>[2x]MKLALNTEFKKAIDLATNSSKNLFITGKAGTGKSTFLKYLINELLFDAVVLAPTGVAAINIGGETIHSFFNFPINITPDKIPDLFIYDYEIYKYVNTIIIDEISMVRADLLDC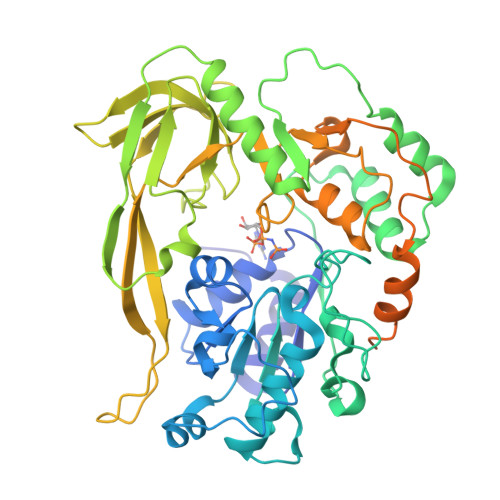IDLFLKRVKNPKLPFGGTKMIFIGDLYQLPPVLTNHQKKAFNMEYESPYFFSAKVFKEMDMEFIEFETIYRQSDKLFIDILNRIRNNTVTDEDIKIINSRVQDKIDNDDGYIYITTVNKKAEEINNQKLDKLKGKLYKLNGTLKGNFDENSLPTPKNLHLKIGAQVMLLNNAPDRMWVNGTIGTITNIFPDEMIIELALENGNIVEITPFKWDMIKFTYDKKEKKMLSETIGSYTQFPLKLAYAITVHKSQGKTFHKVIIDTSRHFFAPGQFYVALSRCTSLDGIILTKKITKNSIILDKKVVNFLTNFQYQLSEKKTPLEEKISILKRAIERNSPLEIVYLKTKDEKSKRVIIPKEVGEMVYSGKSFMGLKGFCTMRNDERVFRIDRILEIKEIND>MQAQITGRPEWIWLALGTALMGLGTLYFLVKGMGVSDPDAKKFYAITTLVPAIAFTMYLSMLLGYGLTMVPFGGEQNPIYWARYADWLFTTPLLLLDLALLVDADQGTILALVGADGIMIGTGLVGALTKVYSYRFVWWAISTAAMLYILYVLFFGFTSK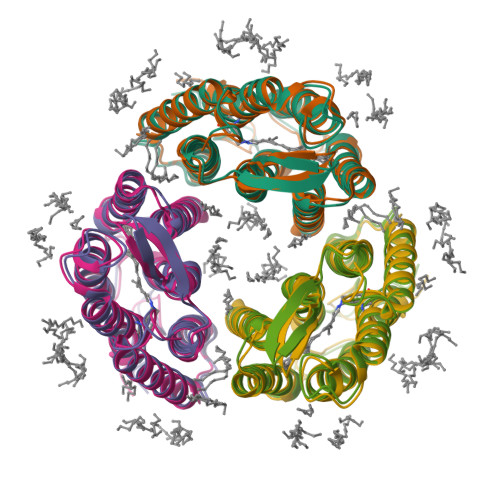AESMRPEVASTFKVLRNVTVVLWSAYPVVWLIGSEGAGIVPLNIETLLFMVLDVSAKVGFGLILLRSRAIFGEAEAPEPSADGAAATS[2x]2-(1-CARBOXY-2-HYDROXY-ETHYL)-5,5-DIMETHYL-THIAZOLIDINE-4-CARBOXYLIC ACID | C9 H15 N O5 S | 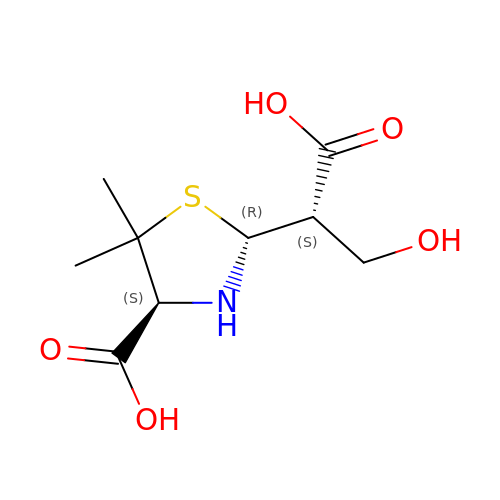NVIIKEPLEZSMNU-NGJCXOISSA-N> MRDTRFPCLCGIAASTLLFATTPAIAGEAPADRLKALVDAAVQPVMKANDIPGLAVAISLKGEPHYFSYGLASKEDGRRVTPETLFEIGSVSKTFTATLAGYALTQDKMRLDDRASQHWPALQGSRFDGISLLDLATYTAGGLPLQFPDSVQKDQAQIRDYYRQWQPTYAPGSQRLYSNPSIGLFGYLAARSLGQPFERLMEQQVFPALGLEQTHLDVPEAALAQYAQGYGKDDRPLRVGPGPLDAEGYGVKTSAADLLRFVDANLHPERLDRPWAQALDATHRGYYKVGDMTQGLGWEAYDWPISLKRLQAGNSTPMALQPHRIARLPAPQALEGQRLLNKTG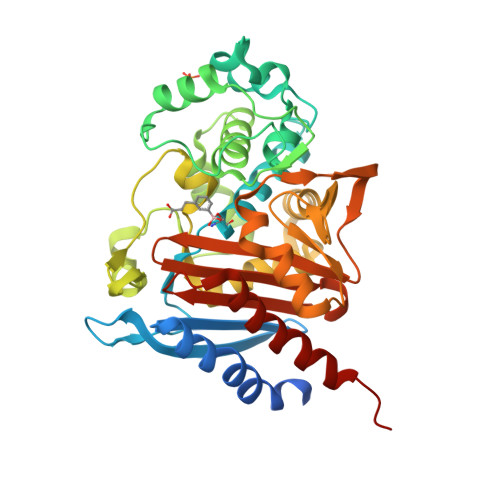STNGFGAYVAFVPGRDLGLVILANRNYPNAERVKIAYAILSGLEQQGKVPLKR>[10x]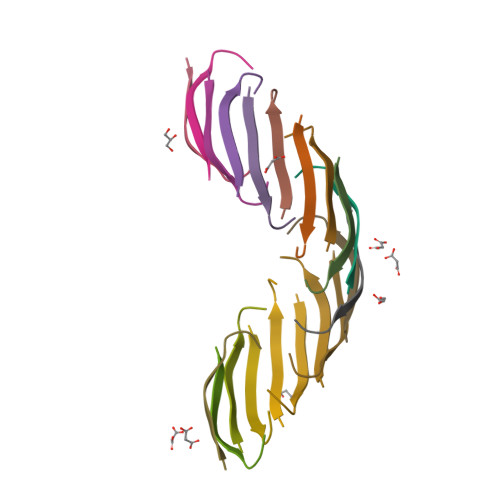KVKVWGSIKRL>MKDLKKIESYLDKLRIKEKDGEERKIYAEVLDGRTLKTLYKLSAKGYITAMGGVISTGKEANVFYADGVFDGKPVAMAVKIYRIETSEFDKMDEYLYGDERFDMRRISPKEKVFIWTEKEFRNLERAKEAGVSVPQPYTYMKNVLLMEFIGEDELPAPTLVELGRELKELDVEGIFNDVVENVKRLYQEAELVHADLSEYNI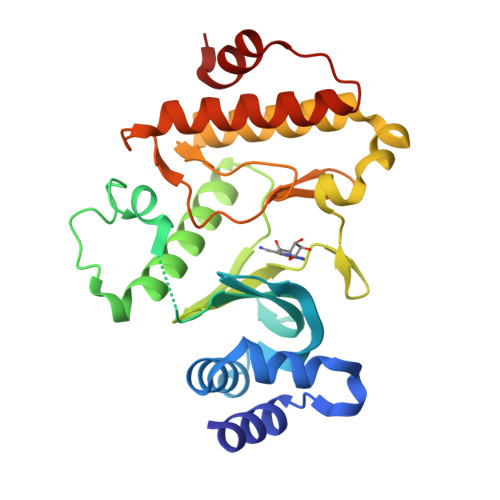MYIDKVYFIDMGQAVTLRHPMAESYLERDVRNIIRFFSKYGVKADFEEMLKEVKGE[2x]>[2x]MKHHHHHHHHGGLVPRGSHGGSEFQVRSFEEIKRSGEIRIGTEGAFPPFNYFDERNQLTGFEVDLG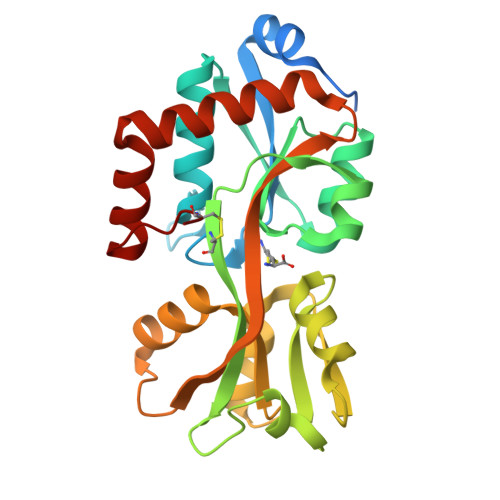NAIAERLGLKPRWIAQSFDTLLIQLNQGRFDFVIASHGITEERARAVDFTNPHYCTGGVIVSRKGGPRTAKDLQGKVVGVQVGTTYMEAAQKIPGIKEVRTYQRDPDALQDLLAGRIDTWITDRFVAKEAIKERKLENTLQVGELVFQERVAMAVAKGNKSLLDALNRALAELMQDGTYARISQKWFGEDVRCK(2S,5R)-1-formyl-N'-[(3R)-piperidine-3-carbonyl]-5-[(sulfooxy)amino]piperidine-2-carbohydrazide 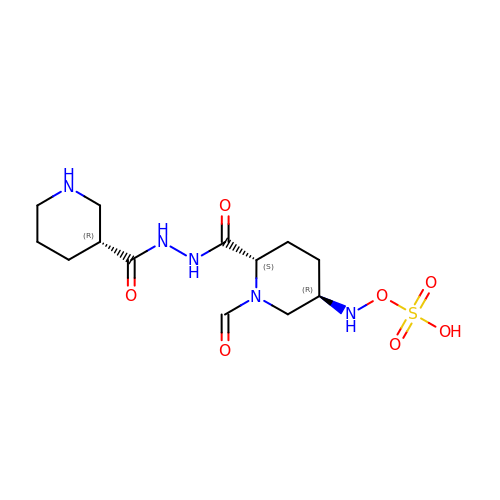| C13 H23 N5 O7 S | KMYLRFCWFBWPGR-MXWKQRLJSA-N>[2x]APQQINDIVHRTITPLIEQQKIPGMAVA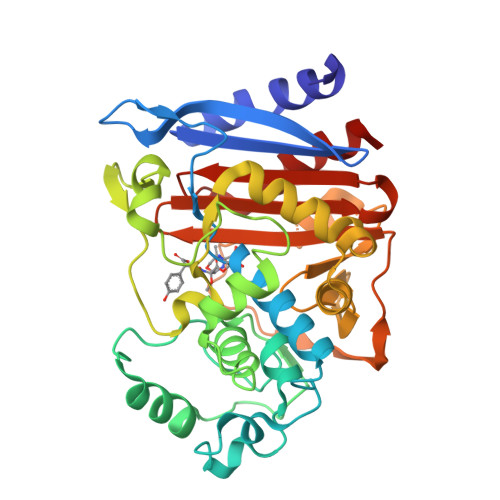VIYQGKPYYFTWGYADIAKKQPVTQQTLFELGSVSKTFTGVLGGDAIARGEIKLSDPTTKYWPELTAKQWNGITLLHLATYTAGGLPLQVPDEVKSSSDLLRFYQNWQPAWAPGTQRLYAASSIGLFGALAVKPSGLSFEQAMQTRVFQPLKLNHTWINVPPAEEKNYAWGYREGKAVHVSPGALDAEAYGVKSTIEDMARWVQSNLKPLDINEKTLQQGIQLAQSRYWQTGDMYQGLGWEMLDWPVNPDSIINGSDNKIALAARPVKAITPPTPAVRASWVHKTGATGGFGSYVAFIPEKELGIVMLANKNYPNPARVDAAWQILNALQ> TD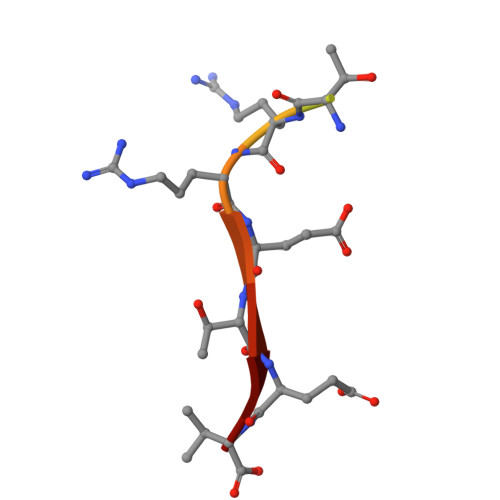DSKPTRRETEV> MAHHHHHHMHIRKERPQDAAEIRQVTEAAFRPVAYSNQKEGEIVDALRAAKALTL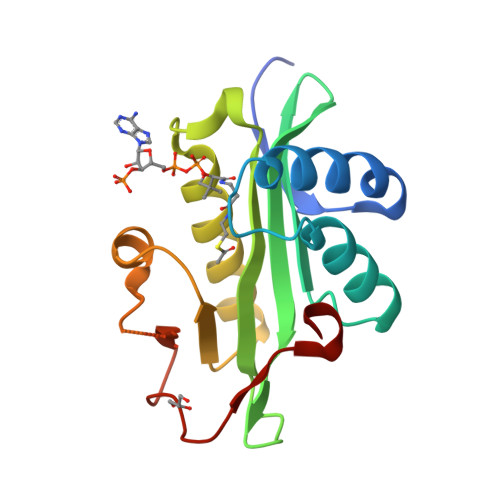SLVAEEDGQVLGHIAFSPVLIGGAEKGWYGLGPVSVLPARQGEGIGGKLIREGLAQLRGAGARGCVLLGDLGYYRRFGFKADARQKLPGVPPEYFQCLAFGPDMPQGDVAYHAAFDA> AQPFAHLTINATDIPSGSHKVSLSSWYHDRGWAKISNMTFSNGKLIVNQDGFYYLYANICFRHHETSGDLATEYLQL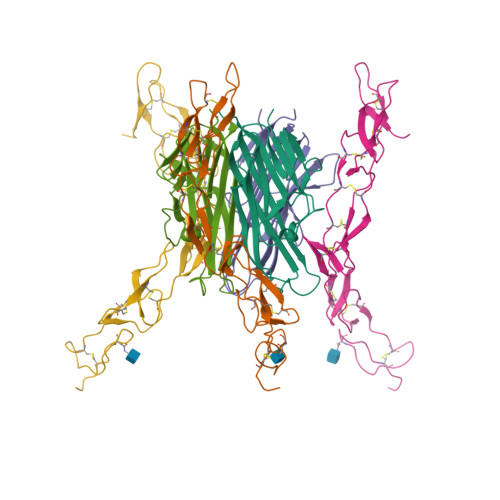MVYVTKTSIKIPSSHTLMKGGSTKYWSGNSEFHFYSINVGGFFKLRSGEEISIEVSNPSLLDPDQDATYFGAFKVRDIDHHHHHH;> ETFPPKYLHYDEETSHQLLCDKCPPGTYLKQHCTAKWKTVCAPCPDHYYTDSWHTSDECLYCSPVCKELQYVKQECNRTHNRVCECKEGRYLEIEFCLKHRSCPPGFGVVQAGTPERNTVCKRCPDGFFSNETSSKAPCRKHTNCSVFGLLLTQKGNATHDNICSHHHHHH>[2x]EAEAEFGACGAIASTVPNYNNAKLPDPFTFANGTALRTKADWSCRRAEISALIQNYEAGTLPPKPPVVTASFSKSGNTGTLAITAGLSNSQTIKFSPTISYPSGTPPANGWPLIIAYEGGSIPIPAGVATLTYSNSDMAQQNSASSRGQGLFYQLYGSTHSASAMTAWVWGVSRIIDALEMTPTAQINTQRIGVTGCARDGKGALMAGAFEERIALTIPQES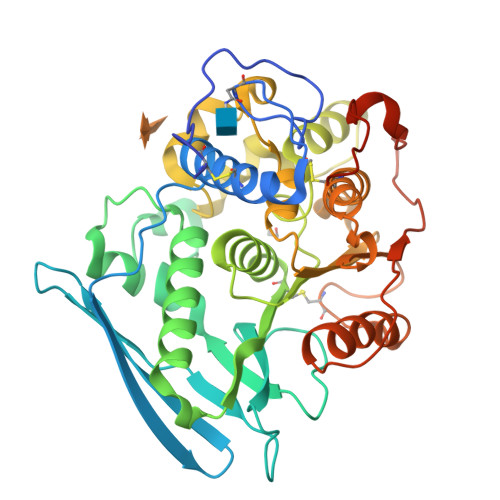GSGGDACWRLSKYEIDNGNQVQDAVEIVGENVWFSTNFNNYVQKLPTVPEDHHLLAAMVAPRAMISFENTDYLWLSPMSSFGCMTAAHTVWQGLGIADSHGFAQVGGHAHCAWPSSLTPQLNAFINRFLLDQSATTNVFTTNNQFGKVQWNAANWITWTTPTLTENLYFQGVDHHHHHH>MNDYSRQNFQDLNLFRGLGEDPAYHPPVLTDRPRDWPLDRWAEAPRDLGYSDFSPYQWRGLRMLKDPDTQAVYHDMLWELRPRTIVELGVYNGGSLAWFRDLTKIMGIDCQVIGIDRDLSRCQIPASDMENITLHQGDCSDLTTFEHLREMAHPLIFIDNAHANTFNIMKWAVDHLLEEGDYFIIEDMIPYWYRYAPQ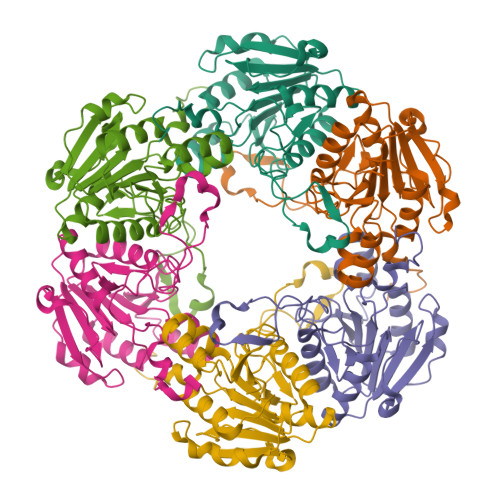LFSEYLGAFRDVLSMDMLYANASSQLDRGVLRRVAAKQ[12x]NA is a homotetrameric transmembrane glycoprotein responsible for cleavage of sialic acid from the host cell membrane. By blocking NA enzymatic activity, neuraminidase inhibitors (NAIs) prevent new viral particles from being released from the surface of an infected cell, thus stopping the spread of virus in the airways. In this study, we applied a set of experimental techniques using recombinant NA variants to understand the molecular basis of development of oseltamivir resistance in the viral N1 neuraminidase NA2009. To decipher the structural mechanism of resistance, we determined crystal structures of NA2009 mutants in complex with oseltamivir carboxylate.

Three variants (H275Y, H275Y/I223V, and H275Y/S247N NA2009) crystallized in the monoclinic space group with four molecules in the asymmetric unit, representing the tetrameric biological unit. Crystal structures of enzymes containing the H275Y substitution either alone or in combination with other mutations show that the bulkier tyrosine side chain pushes the side chain of the neighboring E277 into the binding site, affecting the binding pose of oseltamivir. Specifically, the position of the pentyloxy substituent of oseltamivir changes relative to that in the wt enzyme; the shift in position of the terminal C atom (C91) is more than 2 Å. The crystal structure provides a direct explanation for the more than 1000-fold reduction in binding affinity for oseltamivir in variants containing the H275Y substitution. A similar effect on oseltamivir binding was previously observed for the H275Y substitution in H5N1 avian influenza neuraminidase. Compared to wt, the sensitivity of the H275Y single mutant to oseltamivir decreased considerably (more than 1000-fold increase in Ki). For the H275Y single mutant, the enthalpy change for oseltamivir binding was substantially affected and was 8.7 kcal mol−1 less favorable than the wt value. This change was only partially compensated by a more favorable entropic contribution of 6 kcal mol−1 (referenced to the wt value). The substantial decrease in strength of oseltamivir binding to the H275Y mutant is caused by a significant loss of binding enthalpy, which is partially compensated by a gain in binding entropy. However, we did not confirm the loss of a hydrogen bond between R152 and the oseltamivir acetyl group, which was proposed by Le and co-workers based on molecular dynamics simulations as an additive molecular mechanism conferring drug resistance in H5N1 and H1N1 strains bearing H275Y mutations.

>SVKLAGNSSLCPVSGWAIYSKDNSVRIGSKGDVFVIREPFISCSPLECRTFFLTQGALLNDKHSNGTIKDRSPYRTLMSCPIGEVPSPYNSRFESVAWSASACHDGINWLTIGISGPDNGAVAVLKYNGIITDTIKSWRNNILRTQESECACVNGSCFTVMTDGPSNGQASYKIFRIEKGKIVKSVEMNAPNYYYEECSCYPDSSEITCVCRDNWHGSNRPWVSFNQNLEYQIGYICSGIFGDNPRPNDKTGSCGPVSSNGANGVKGFSFKYGNGVWIGRTKSISSRNGFEMIWDPNGWTGTDNNFSIKQDIVGINEWSGYSGSFVQHPELTGLDCIRPCFWVELIRGRPKENTIWTSGSSISFCGVNSDTVGWSWPDGAELPFTIDK[4x]>[2x]AEETCFDKYTGNTYRVGDTYERPKDSMIWDCTCI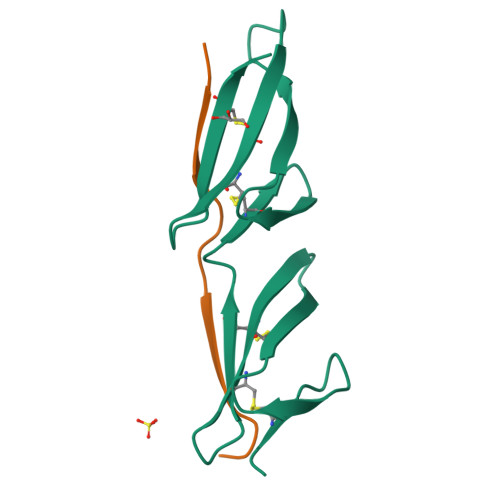GAGRGRISCTIANRCHEGGQSYKIGDTWRRPHETGGYMLECVCLGNGKGEWTCKPI;>[2x]XTGMSGFSETVTIVEDTRPX2-{1-[2-(piperidin-1-yl)ethyl]-1H-benzimidazol-2-yl}thieno[3,2-b]pyridine-7-carboxylic acid | C22 H22 N4 O2 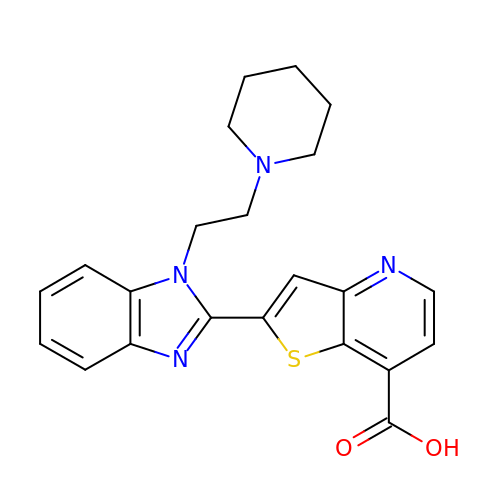S | FUHPYFIFOFNOHS-UHFFFAOYSA-N>[4x]GADAAPQLGKRKRELDVEEAHAASTEEKEA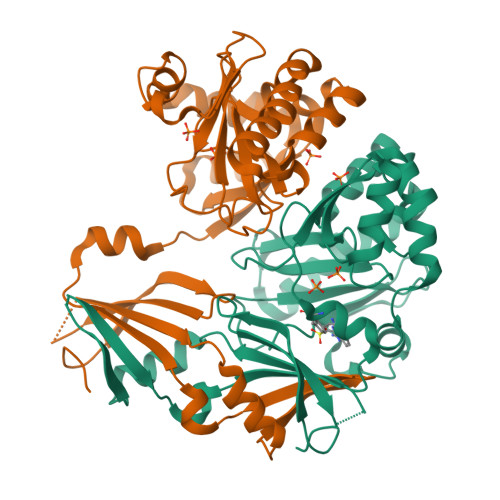GVGNGTCAPVRLPFSGFRLQKVLRESARDKIIFLHGKVNEASGDGDGEDAVVILEKTPFQVEQVAQLLTGSPELQLQFSNDIYSTYHLFPPRQLNDVKTTVVYPATEKHLQKYLRQDLRLIRETGDDYRNITLPHLESQSLSIQWVYNILDKKAEADRIVFENPDPSDGFVLIPDLKWNQQQLDDLYLIAICHRRGIRSLRDLTPEHLPLLRNILHQGQEAILQRYRMKGDHLRVYLHYLPSYYHLHVHFTALGFEAPGSGVERAHLLAEVIENLECDPRHYQQRTLTFALRADDPLLKLLQEAQQS> GSMLDDNRPMDFAKDKNSATLWAKKRKQVWLNNLSKAESTSINNYIKNSSEINSYSIKKKFALDNYEGIETLNEDLKNISTAVKKSMLTKPLYVYYYEANDKFGFNQNLESSLDSNIIDEEAINNFAKKISDTNFIQDGFKDVTMTEPDINSKLPILVHLKLP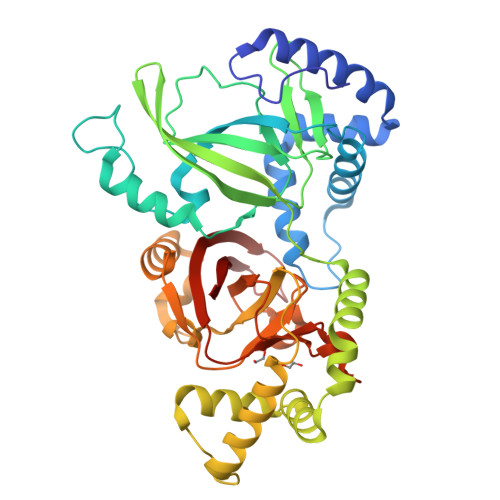TNTPAASYGNDEENLRVLIDQGYSLKATGLSIVTIKGKQYAKVDADLIKQLNFENDVISASQWGEENYAPWLKELTSNELRDINNYLGGGYTAINKYLLDGTIGENTSKEDLEEKISNISSALKKRKIPEDIITYRRMGPNEFGLDLNSPDYDFNKVENVSKFKEKWLGKTIPVKTFISTTVLSNNISAFAKRKLILRLHLPNGSNAAYVSVAEGYKNEYEVLIDHGYSYKIDNITEYYDESSLGGKTNKLIIDATLI> RPPNIVLIFADDLGYGDLGCYGHPSSTTPNLDQLAAGGLRFTDFYVPVSLSTPSRAALLTGRLPVRMGMYPGVLVPSSRGGLPLEEVTVAEVLAARGYLTGMAGKWHLGVGPEGAFLPPHQGFHRFLGIPYSHDQGPCQNLTCFPPATPCDGGCDQGLVPIPLLANLSVEAQPPWLPGLEARYMAFAHDLMADAQRQDRPFFLYYASHHTHYPQFSGQSFAERSGRGPFGDSLMELDAAVGTLMTAIGDLGLLEETLVIFTADNGPETMRMSRGGCSGLLRCGKGTTYEGGVREPALAFWPGHIAPGVTHELASSLD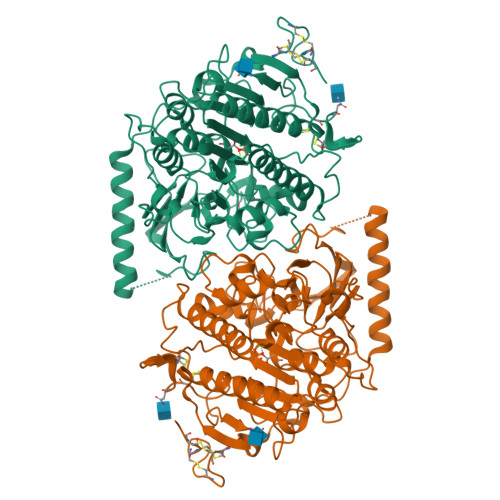LLPTLAALAGAPLPNVTLDGFDLSPLLLGTGKSPRQSLFFYPSYPDEVRGVFAVRTGKYKAHFFTQGSAHSDTTADPACHASSSLTAHEPPLLYDLSKDPGENYNLLGGVAGATPEVLQALKQLQLLKAQLDAAVTFGPSQVARGEDPALQICCHPGCTPRPACCHCPDPHA The long-wavelength beamline I23 at Diamond Light Source overcomes these limitations and extends the accessible wavelength range to λ = 5.9 Å. In this study, we report the determination of diverse protein structures by experimental phasing techniques carried out at long wavelengths on beamline I23 at Diamond Light Source using S, Ca, K, Cl, V, I, Cd, and P as anomalous scatterers. Native-SAD uses light atoms naturally occurring in proteins or bound to proteins. We demonstrate that long-wavelength native-SAD has become a very compelling technique, where a low multiplicity dataset from a single crystal can be sufficient for successful structure determination, making it a general vehicle of choice for experimental phasing.

Using this protocol, we selected 10 projects solved by S-SAD phasing at the beamline, including soluble and membrane proteins. Structures varied in size with molecular weights ranging from 14 to 114 kDa, sulfur contents varied between 0.9 and 6.5%, and diffraction resolution from 1.8 (detector limited) to 3.4 Å. The overall multiplicity for these datasets was below 26, which is four times lower than the multiplicity typically needed for S-SAD at shorter wavelengths (100)10.

> MPAHSLVMSSPALPAFLLCSTLLVIKMYVVAIITGQVRLRKKAFANPEDALRHGGPQYCRSDPDVERCLRAHRNDMETIYPFLFLGFVYSFLGPNPFVAWMHFLVFLVGRVAHTVAYLGKLRAPIRSVTYTLAQLPCASMALQILWEAARHL> MRITQGTFSFLPELTDEQITKQLEYCLNQGWAVGLEYTDDPHPRNTYWEMFGLPMFDLRDAAGILMEINNARNTFPNHYIRVTAFDSTHTVESVVMSFIVNRPADEPGFRLVRQEEPGRTL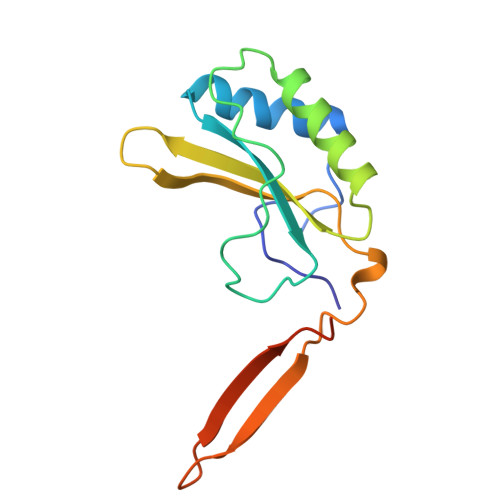RYSIESYAVQAGPEGSRY> TIA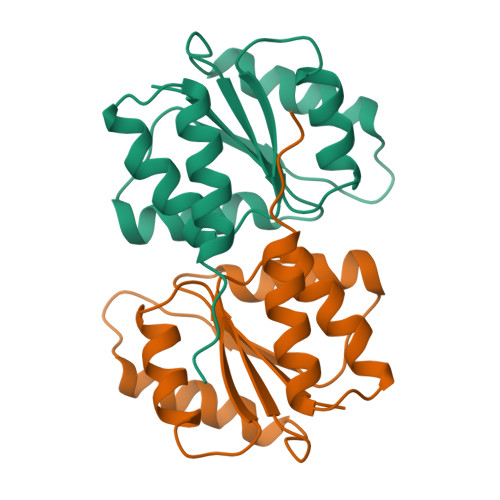IVIGTHGWAAEQLLKTAEMLLGEQENVGWIDFVPGENAETLIEKYNAQLAKLDTTKGVLFLVDTWGGSPFNAASRIVVDKEHYEVIAGVNIPMLVETLMARDDDPSFDELVALAVETGREGVKALKAKPFAG>MPKPYVAINMAELKNEPKTFEMFASVGPKVCMVTARHPGFVGFQNHIQIGILPFGNRYGGAKMDMTKESSTVRVLQYTFWKDWKDHEEMHRQNWSYLFRLCGSCASQMIWGPWEPIYEIIYANMPINTEMTDFTAVVGKKFAEGKPLDIPVISQPYGKRVVAFAEHSVIPGKEKQFEDAIVRTLEMLKKAPGFLGAMVLKEIGVSGIGSMQFGAKGFHQVLENPGSLEPDPNNVMYSVPEAKNTPQQYIVHVEWANTDALMFGMGRVLLYPELRQVHDEV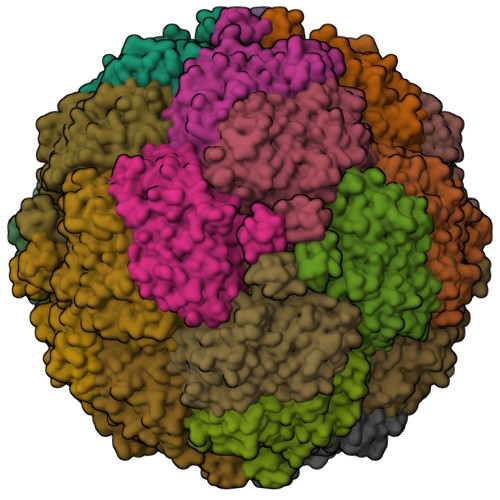LDTLVYGPYIRILNPMMEGTFWREYLNENAWRHPQFGG[6x]>[2x]MDFTKPETVLNLQNIRDELVRMEDSIIFKFIERSHFATCPSVYEANHPGLEIPNFKGSFLDWALSNLEIAHSRIRRFESP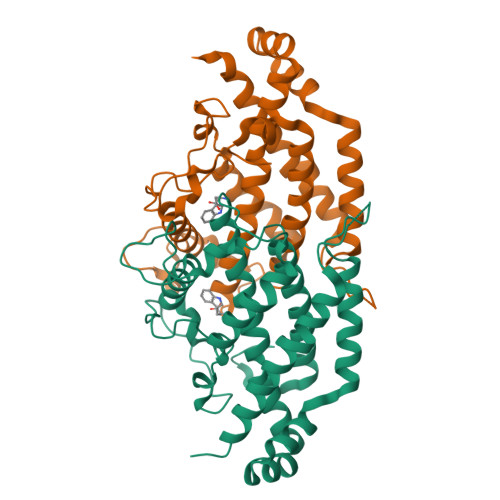DETPFFPDKIQKSFLPSINYPQILAPYAPEVNYNDKIKKVYIEKIIPLISKRDGDDKNNFGSVATRDIECLQSLSRRIHFGKFVAEAKFQSDIPLYTKLIKSKDVEGIMKNITNSAVEEKILERLTKKAEVYGVDPTNESGERRIIPEYLVKIYKEIVIPITKEVEVEYLLRRLEE N-[(furan-2-yl)methyl]-5,6,7,8-tetrahydro[1]benzothieno[2,3-d]pyrimidin-4-amine | C15 H15 N3 O S | 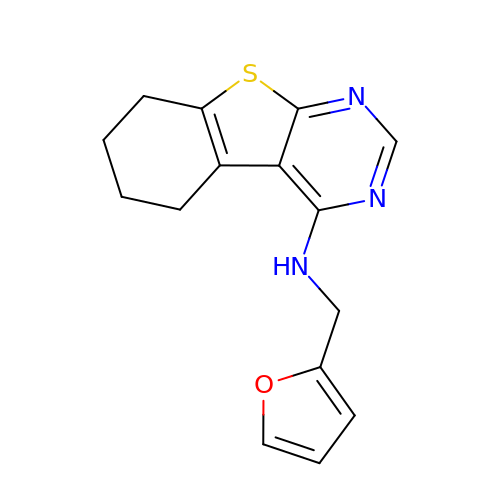OZBAWCPXMIEVSW-UHFFFAOYSA-N(2S,5S)-hexane-2,5-diol | C6 H14 O2 | 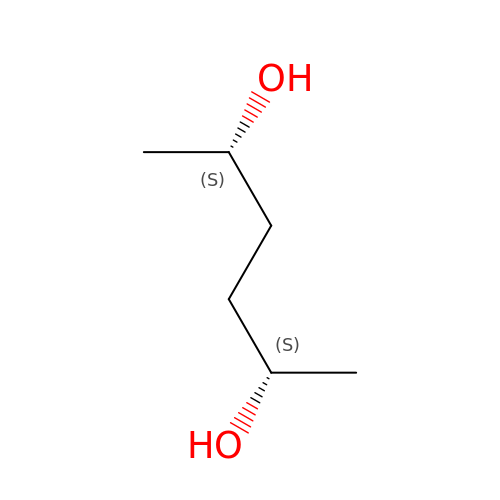OHMBHFSEKCCCBW-WDSKDSINSA-N>[33x]MAVNVNTNVAAM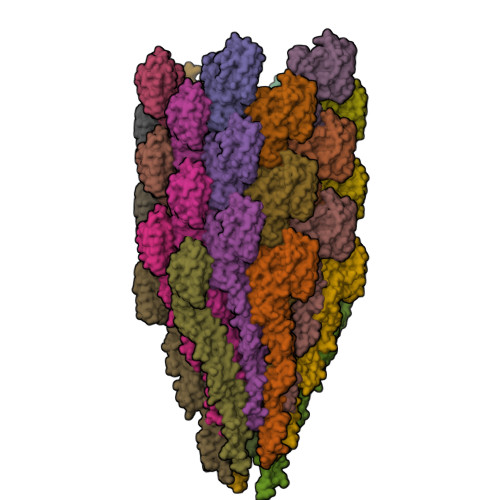TAQRYLTGATNAQQTSMERLSSGFKINSAKDDAAGLQISNRLNVQSRGLDVAVRNANDGISIAQTAEGAMNETTNILQRMRDLSLQSANGSNSKSERVAIQEEITALNDELNRIAETTSFGGNKLLNGTFSTKSFQIGADNGEAVMLTLKDMRSDNRMMGGTSYVAAEGKDKDWKVQAGANDITFTLKDIDGNDQTITVNAKEGDDIEEVATYINGQTDMVKASVNEKGQLQIFAGNNKVTGDVAFSGGLAGALNMQAGTAETVDTIDVTSVGGAQQSVAVIDSALKYVDSHRAELGAFQNRFNHAISNLDNINENVNASKSRIKDTDFAKETTALTKSQILSQASSSVLAQAKQAPNAALSLLG> MSTLFPKYSKTTDGSKVIMEQRLLQQVNNLILDNDICTGCGICSEVCPEEAISVGAVGGVRRGLVDDAASIHVDETKCSYCGVCVIMCPFSALALKVDGEERLPILEKEGFPTYDKGT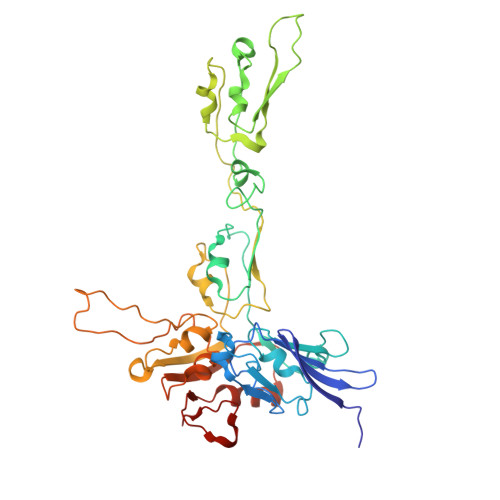AIDQDKCVRCNICDDVCPRDAIDRDVPLFEGEDKEGLAKGQAVELKIEFKVDDEKCTKCGICGNLCEAINVLHKPFSPEIGKVEGEVIWDEAYCDGCNVCAEACPSEAIKVTRTVVGQKKLGNVNIIDEDCCTCRWCAINCPTEAITVNKIFEGEITFHAEKCPGGCSTCVDVCPANAIYLPTPKPAKDMKGQIEAKIAVNKDFCILCGACVNACPGEDIIYLRRDSVKIKGKETDLFKKIKEKLFTPRTSKVKEQPSLAGSVELKAVSQ> MDGSGEQPRGGGPTSSEQIMKTGALLLQGFIQDRAGRMGGEAPELALDPVPQDASTKKLSESLKRIGDELDSNMELQRMIAAVDTDSPREVFFRVAADMFSDGNFNWGRVVALFYFASKLVLKALSTKVPELIRTIMGWTLDFLRERLLGWIQDQGGWDGLLSYGSS;> DMRPEIWIAQELRRIGDEFN

The intrinsic pathway to apoptosis is regulated by interactions between members of three factions of the Bcl-2 protein family: the BH3-only proteins such as Bim and Bid, which initiate the process, the essential effectors Bax and Bak, and the prosurvival members, which oppose the action of both other factions. Unlike Bak, which is constitutively anchored in the mitochondrial outer membrane (MOM) via its C-terminal segment, Bax is largely cytosolic in healthy cells and accumulates at the MOM only upon a death signal. Core/latch dimers of Bax and Bak form on treatment of the monomeric proteins with certain BH3 peptides and CHAPS, and Bax and Bak core domains form symmetric homodimers, supporting that unlatching the core domain is a necessary step to Bax and Bak oligomerisation and permeabilisation of the MOM. Bim and Bid are both potent direct activators of Bax, but Bim is less dependent on interactions via its ‘h0' residues than is Bid.

To explore the consequences of removing α8, presumably an early event in separation of the core and latch domains, we crystallised the BimBH3mini:BaxΔC28 complex and determined its structure. C-terminal truncations that remove more of α8 cannot be expressed. The loss of the cavity in BimBH3mini:BaxΔC28 complex through movement of α2 demonstrates that the positions of α2 and α8 are coupled, but sheds little additional light on the unfolding pathway of unlatching. Removal of helix 8 at some stage during Bax activation is clearly a requirement of our hypothesis that the core domain must be unlatched to allow oligomerisation.> MENDMKSLSAAAQACVKKMRDAKVNEACIRTFIAQHVMVSKGETGSIPDSAIMPVDSLDALDSLTIECDNAVLQSTVVLKLNGGLGTGMGLCDAKTLLEVKDGKTFLDFTALQVQYLRQHCSEHLRFMLMDSFNTSASTKSFLKARYPWLYQVFDSEVELMQNQVPKILQDTLEPAAWAENPAYEWAPPGHGDIYTALYGSGKLQELVEQGYRYMFVSNGDNLGATIDKRVLAYMEKEKIDFLMEVCRRTESDKKGGHLARQTVYVKGKDGQPDAEKRVLLLRESAQCPKADMESFQDINKYSFFNTNNLWIRLPVLLETMQEHGGTLPLPVIRNEKTVDSSNSASPKVYQLETAMGAAIAMFESASAIVVPRWRFAPVKTCADLLALRSDAYVVTDDFRLVLDDRCHGHPPVVDLDSAHYKMMNGFEKLVQHGVPSLVECKRVTVKGLVQF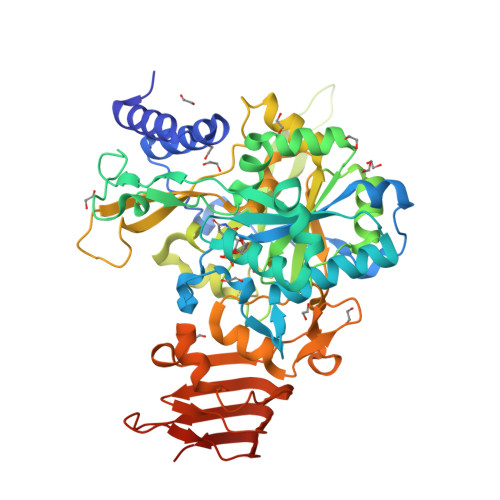GAGNVLTGTVTIENTDSASAFVIPDGAKLNDTTASPQQSTNKMRPLEHHHHHH>MASFGSRMEESIRKTVTENTVVIYSKTWCSYCTEVKTLFKRLGVQPLVVELDQLGPQGPQLQKVLERLTGQHT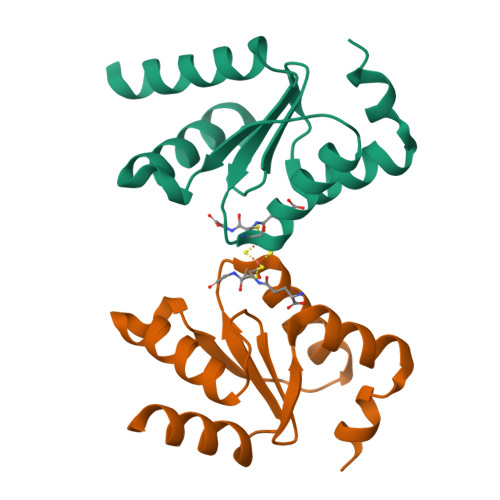VPNVFVCGKHIGGCTDTVKLNRKGDLELMLAEANGKNGQS[2x]>[2x]DPGTIVHNFSRTEPRTEPAGGSHSGSSSKLQALFAHPLYNVPEEPPLLGAEDSLLASQEALRYYRRKVARWNRRHKMYREQMNLTSLDPPLQLRLEASWVQFHLGINRHGLYSRSSPVVSKLLQDMRHFPTISADYSQDEKALLGACDCTQIVKPSGVHLKLVLRFSDFGKAMFKPMRQQRDEETPVDFFYFIDFQRHNAEIAAFHLDRILDFRRVPPTVGRIVNVTKEILEVTKNEILQSVFFVSPASNVCFFAKCPYMCKTEYAVCGKPHLLEGSL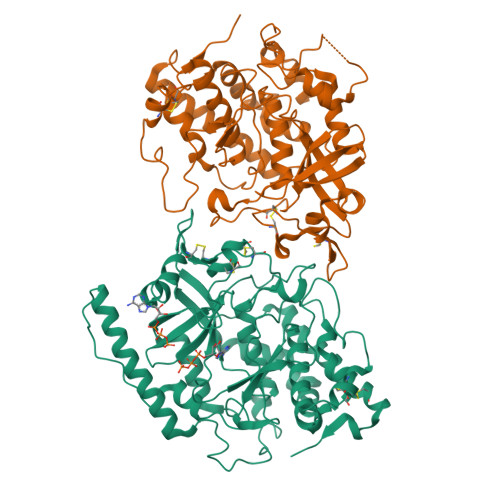SAFLPSLNLAPRLSVPNPWIRSYTLAGKEEWEVNPLYCDTVKQIYPYNNSQRLLNVIDMAIFDFLIGNMDRHHYEMFTKFGDDGFLIHLDNARGFGRHSHDEISILSPLSQCCMIKKKTLLHLQLLAQADYRLSDVMRESLLEDQLSPVLTEPHLLALDRRLQTILRTVEGCIVAHGQQSVIVDGPVEQ;>RDPGPRRSESPPGPGGDASLLARLFEHPLYRVAVPPLTEEDVLFNVNSDTRLSPKAAENPDWPHAGAEGAEFLSPGEAAVDSYPNWLKFHIGINRYELYSRHNPAIEALLHDLSSQRITSVAMKSGGTQLKLIMTFQNYGQALFKPMKQTREQETPPDFFYFSDYERHNAEIAAFHLDRILDFRRVPPVAGRMVNMTKEIRDVTRDKKLWRTFFISPANNICFYGECSYYCSTEHALCGKPDQIEGSLAAFLPDLSLAKRKTWRNPWRRSYHKRKKAEWEVDPDYCEEVKQTPPYDSSHRILDVMDMTIFDFLMGNMDRHHYETFEKFGNETFIIHLDNGRGFGKYSHDELSILVPLQQCCRIRKSTYLRLQLLAKEEYKLSLLMAESLRGDQVAPVLYQPHLEALDRRLRVVLKAVRDCVERNGLHSVVDDDLDTEH[2x]> KEYDAYLSYTKVDQDTLDCDNPEEEQFALEVLPDVLEKHYGYKLFIPERDLIPSGTYMEDLTRYVEQSRRLIIVLTPDYILRRGWSIFELESRLHNMLVSGEIKVILIECTELKGKVNCQEVE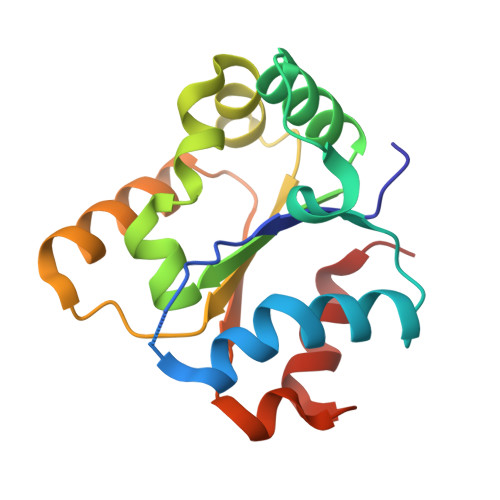SLKRSIKLLSLIKWKGSKSSKLNSKFWKHLVYEMPIK>MAHHHHHHMSIIEFWLEAKATIDRLIEQFLNSNRDWDLVDISSYILKDGKRFRGTLNMFFTVALGGDIKDSYGGALAIEILHSASLALDDIVDLDATRRGDKAAWVVYGNRKVIFITNYLIPTALRIIQTSYGDDALNTSIELEKDTSVGALRDMYDNSDYIRTIELKTGS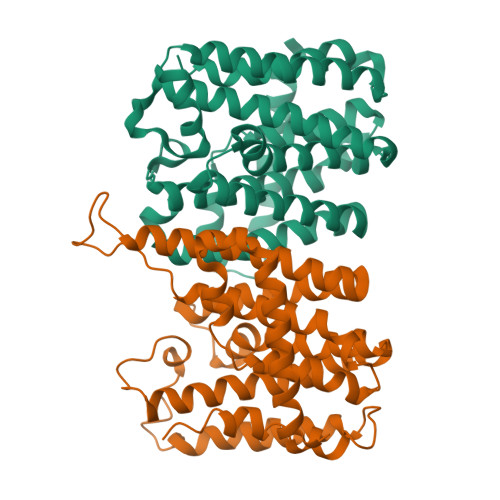LFKLSTVLSAYASKHYNTKQQMLDVGKYLGIIYQVIDDFVDYKTKKVEEIDGSAKQLFKYYREGKLEEYVRSVYLEYKQKYDELISNIPFQSKYLSEIRSLPEFLANGLLKEANIDKI[2x]>MGSSH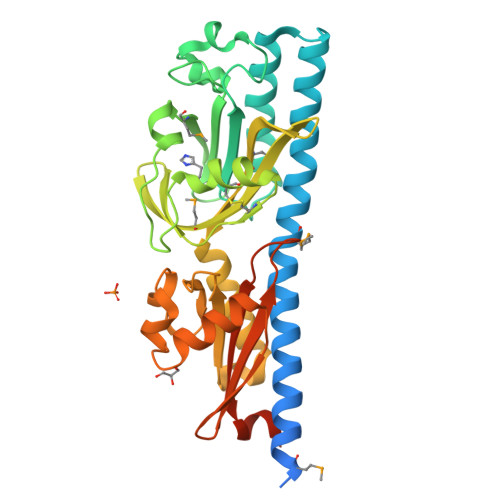HHHHHSSGLVPRGSHQHSSVLVKSASTQMLDESARLRLEARGELQALRIQRYFMDAFQYGKGFSRQILFLRDQAQKRFLDAYDLREDLTRQVRTALAANPEVLGLYVVFEPNALDGKDELFVDQPALGSNDKGRFSLYWAQATPGQLESESMIESELADTSSGPSGAAYNAWYTCPKESGQPCVLDPYFDKVGERQLLMTSIAFPLELDGKVIGVMGLDINLSNLQALSEQGNRELYDGVGQVGILSPAGLFAGNSRDAGLLGKNLAKADPQHAGELLQLLAAGKSRLFNENDDLKVLQPLQPIPGAKPWGVLLEVPKSALLGPALALERQLDDMRREGT[4x]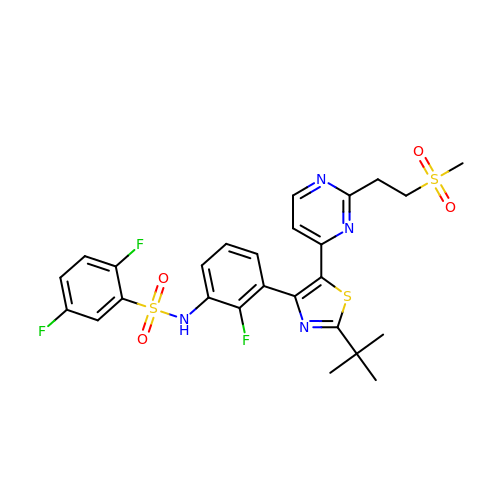N-[3-(2-tert-butyl-5-{2-[2-(methanesulfonyl)ethyl]pyrimidin-4-yl}-1,3-thiazol-4-yl)-2-fluorophenyl]-2,5-difluorobenzene-1-sulfonamide | C26 H25 F3 N4 O4 S3 | JZYMCONNLXIIJS-UHFFFAOYSA-N> MAYVLDTNVAIHLRDG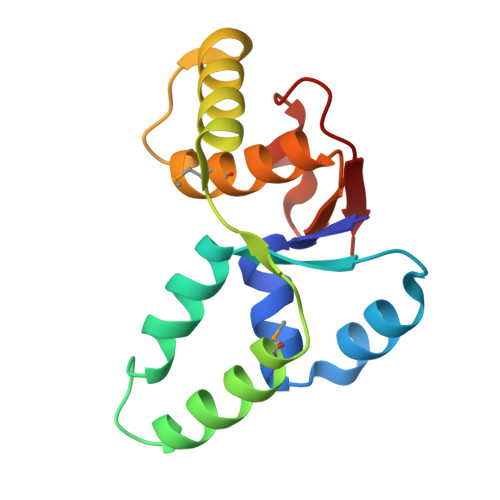DPEVTTRVTALNGAILLSIISRVELEGGVYREAAQAGLRRSRLDVMLKVLPVLDFDGAAADEYRRIVESAGYSRRKVVDRMIAAQALAHRATFVTFNADDFRDIPGLSLLAW>MRGSHHHHHHGSIEGRSAVTCDDYYYGFGCNKFCRPRDDFFGHYACDQNGNKTCMEGWMGPECNRAICRQGCSPKHGSCKLPGDCRCQYGWQGLYCDKCIPHPGCVHGICNEPWQCLCETNWGGQLCDKDL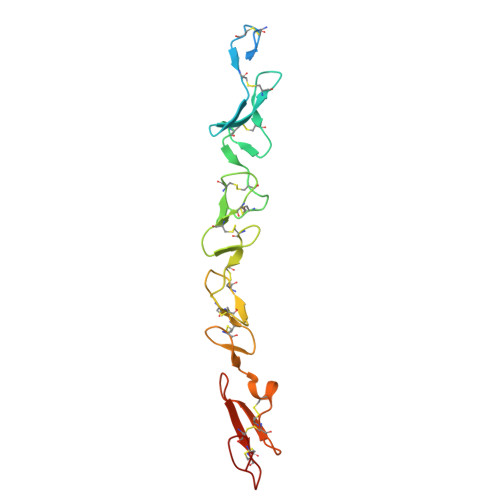NYCGTHQPCLNGGTCSNTGPDKYQCSCPEGYSGPNCEI[2x]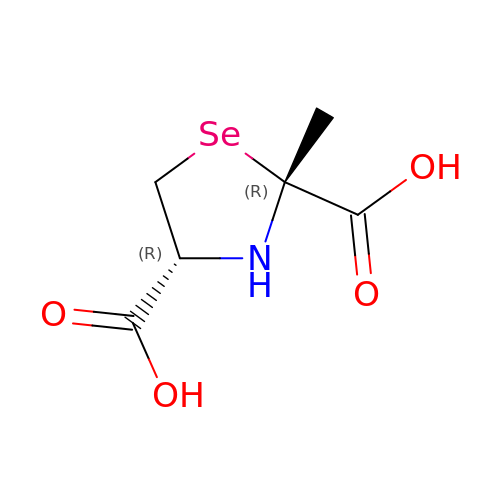(2~{R},4~{R})-2-methyl-1,3-selenazolidine-2,4-dicarboxylic acid | C6 H9 N O4 Se | YQSKWMPEENRPTH-BBIVZNJYSA-N5-acetamido-2,6-anhydro-4-carbamimidamido-3,4,5-trideoxy-7-O-methyl-D-glycero-D-galacto-non-2-enonic acid | C13 H22 N4 O7 | 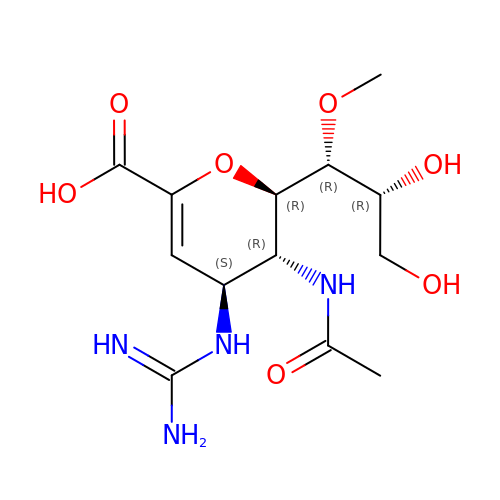QNRRHYPPQFELSF-CNYIRLTGSA-N> PTHYSVALQYDENKMSAPKVVAKGAG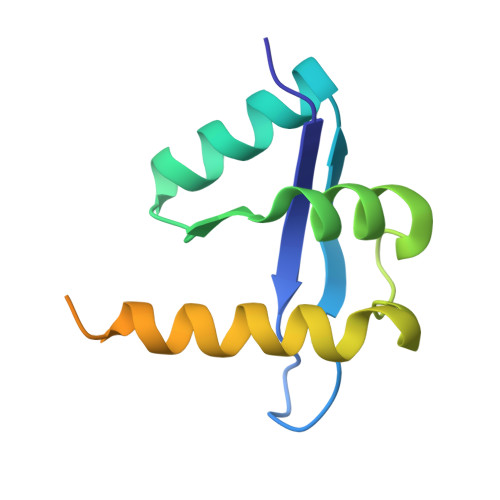LIALRIREIGAEHRVPTLEAPPLARALYRHAEIGQQIPGQLYAAVAEVLAWVWQLKRWRLAGGQRPPQPENLPVPEALDFMNEKNTDA> LKALAYEGEPHEIAENFKKQGNELYKAKRFKDARELYSKGLAVECEDKSINESLYANRAACELELKNYRRCIEDCSKALTINPKNVKCYYRTSKAFFQLNKLEEAKSAATFANQRIDPENKSILNMLSVIDRKEQELKAKEEKQQREAQERENKKIMLESAMTLRNITNIKTHSPVELLNEGKIRLEDPMDFESQLIYPALIMYPTQDEFDFVGEVSELTTVQELVDLVLEGPQERFKKEGKENFTPKKVLVF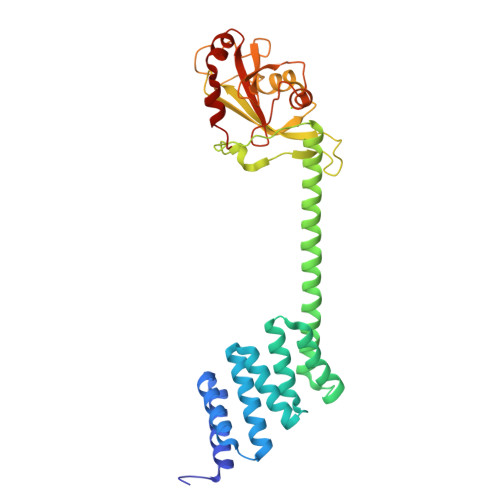METKAGGLIKAGKKLTFHDILKKESPDVPLFDNALKIYIVPKVESEGWISKWDKQKALERRSV>[2x]AKDFSGAELYTLEEVQYGKFEAR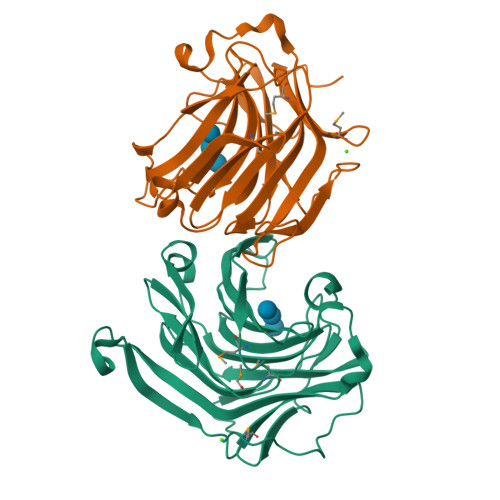MKMAAASGTVSSMFLYQNGSEIADGRPWVEVDIEVLGKNPGSFQSNIITGKAGAQKTSEKHHAVSPAADQAFHTYGLEWTPNYVRWTVDGQEVRKTEGGQVSNLTGTQGLRFNLWSSESAAWVGQFDESKLPLFQFINWVKVYKYTPGQGEGGSDFTLDWTDNFDTFDGSRWGKGDWTFDGNRVDLTDKNIYSRDGMLILALTRKGQESFNGQVPRDD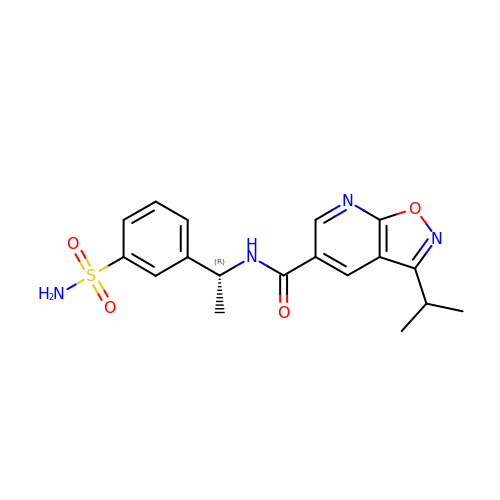3-propan-2-yl-~{N}-[(1~{R})-1-(3-sulfamoylphenyl)ethyl]-[1,2]oxazolo[5,4-b]pyridine-5-carboxamide | C18 H20 N4 O4 S | HRWBSXDFUWMVHN-LLVKDONJSA-N> MADYKDDDDKSGPDEVDASGRMDQNQHLNKTAEAQPSENKKTRYCNGLKMFLAALSLSFIAKTLGAIIMKSSIIHIERRFEISSSLVGFIDGSFEIGNLLVIVFVSYFGSKLHRPKLIGIGCFIMGIGGVLTALPHFFMGYYRYSKETNINSSENSTSTLSTCLINQILSLNRASPEIVGKGCLKESGSYMWIYVFMGNMLRGIGETPIVPLGLSYIDDFAKEGHSSLYLGILNAIAMIGPIIGFTLGSLFSKMYVDIGYVDLSTIRITPTDSRWVGAWWLNFLVSGLFSIISSIPFFFLPQTPNKPQKERKASLSLHVLETNDEKDQTANLTNQGKNITKNVTGFFQSFKSILTNPLYVMFVLLTLLQVSSYIGAFTYVFKYVEQQYGQPSSKANILLGVITIPIFASGMFLGGYIIKKFKLNTVGIAKFSCFTAVMSLSFYLLYFFILCENKSVAGLTMTYDGNNPVTSHRDVPLSYCNSDCNCDESQWEPVCGNNGITYISPCLAGCKSSSGNKKPIVFYNCSCLEVTGLQNRNYSAHLGECPRDDACTRKFYFFVAIQVLNLFFSALGGTSHVMLIVKIVQPELKSLALGFHSMVIRALGGILAPIYFGALIDTTCIKWSTNNCGTRGSCRTYNSTSFSRVYLGLSSMLRVSSLVLYIILIYAMKKKYQEKDINASENGSVMDEANLESLNKNKHFVPSAGADSETHC

OATP1B1, encoded by SLCO1B1 and formerly known as SLC21A6, LST-1, OATP-C, or OATP2, is specifically expressed on the basolateral membrane of hepatocytes. OATP1B1 plays a vital role in mediating the uptake of endogenous compounds such as bile acids, bilirubin, steroid conjugates, and thyroid hormones, as well as a large variety of clinical drugs including statins, antibiotics, antivirals, and anticancer medications for hepatic clearance. The overall architecture of OATP1B1 is composed of the transmembrane domain (TMD) and extracellular loops (ELs) with both N- and C-terminal ends situated in the cytoplasm. The interface between NTD and CTD of OATP1B1 forms a conserved cavity in which substrates bind.

We determined the structures of OATP1B1-apo/B/S/D in outward-open state at resolutions ranging from 2.9 Å to 3.7 Å. Structures of OATP1B1 bound with bilirubin, simeprevir and DCF, adopt similar outward-open conformations as that of OATP1B1-apo. The root mean square deviation between OATP1B1-apo and each of the ligand-bound states is 0.51 Å (apo vs bilirubin), 0.46 Å (apo vs simeprevir), and 0.89 Å (apo vs DCF), respectively. In outward-open OATP1B1-apo/B/S/D, the intracellular gate is closed mainly by TM4 and TM10. A conserved salt bridge is formed by the interaction between D198 and K568. Additionally, multiple hydrophobic residues act as barriers, blocking the intracellular central pathway. Particularly, the ICH is attached to the C-terminus of TM2 through hydrophobic interactions between F325 and aromatic residues, F83, Y86 and F87. This attachment potentially contributes to the sealing and maintenance of the intracellular gate in the outward state. MD simulations support the stable existence of both D198–K568 salt bridge and Y86–F325 hydrophobic interaction in outward-open OATP1B1-apo/B/S/D.>[8x]MSISISYSTTYSGWTVADYLADWSAYFGDVNHRPGQVVDGSNTGGFNPGPFDGSQYALKSTASDAAFIAGGDLHYTLFSNPSHTLWGKLD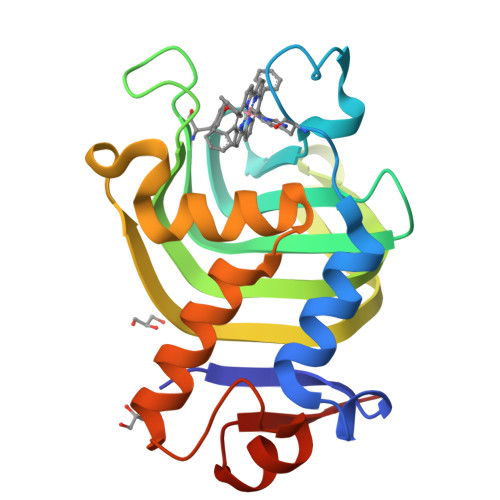SIALGDTLTGGASSGGYALDSQEVSFSNLGLDSPIAQGRDGTVHKVVYGLMSGDSSALQGQIDALLKAVDPSLSINSTFDQLAAAGVAHATPAA>[2x]MHHHHHHSSGRENLYFQGKESGIELPSLANAIENMRKFQNSQKLAQAALLYMASKLTSQEETKELTDIFRHIDKNGDGQLDRQELIDGYSKLSGEEVAVFDLPQIESEVDA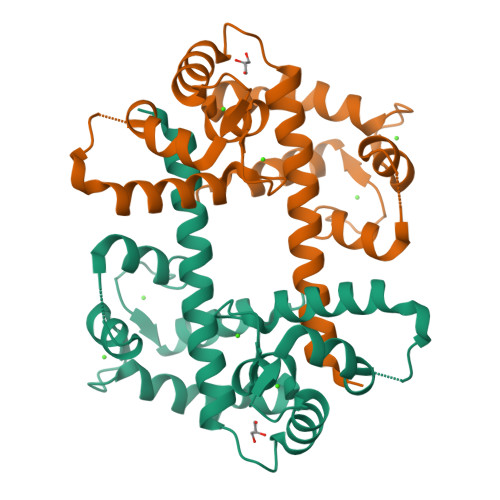ILGAADFDRNGYIDYSEFVTVAMDRKSLLSKDKLESAFQKFDQDGNGKISVDELASVFGLDHLESKTWKEMISGIDSNNDGDVDFEEFCKMIQKLCSNNEPQL> GAMEADLSEPFSLTEVQTAYMLGRNPQFELSGISPQTYFEYETELDIARLSRSFQKVIQRHPMLRAVILPEGKQQILRDVPEYEIEVESLVSMPPEKQAARLREERSRMIDHVFPLGQWPLFELKAFQLQEHTYLLCFRYDALLMDGASMNLVGQDLMHYYHQPDAQLPPLSFTFQDYMHIYDDMKRGTEYETAKAYWTNKLPDFPPAPSLLLAKDPAEIGTPNFQSLTTIITKDKWLKLRRLAQDKQVTPSALLCTVYGEVLAFWSNQRRLAINLTVFNRYPVHDEVEQIVGDFTSLILLDMDMDQKQPFFTKVEQTQSTLLDGLEHRHYDGVEFIRDYTRYHQMRPKAVMPIVFTSMLAGAGAFAWEEIGSLRHIHARTPQVYLDNVVIEKNGELLVSWNYVEELFDAEVMESMFTQFVELLDQLVEQGDINPLRISQKDYALIDQYNATAEPIPAATLHQLFIDQAQRTPDQVAVVFEQEWLTYSELDQRSNQVARFLQSRGIGRGDRVGVLAKRQVETIINLMAVLKAGAAYVPIDPDHPYERQTYILENSSCKILLDSDLYETMEISSYADGDLTPVAEPEDTAYVIYTSGSTGRPKGVIITHQAASNTIQDINRKFEVNEEDRIIGISSMCFDLSVYDIFGTLSAGATLVMIRDPRDMRELVRTVERRGITIWNTVPAIMDLALDHVGSHFENISLRLVLLSGDWIPLPLPAKINRHFPVADVISLGGATEASIWSIYWPIEQVEANWKSIPYGKPLANQTYYVLNYDQKMCPVGVIGDLYIGGAGLAQGYLNDDQKTKDAFIMHPEFGPIYKTGDCGRMRPEGYIEFLGRQDYQVKIQGYRVELEEISHCLLTYPDVDQAVVIDQTDERGMKFLVGYVVAQQEIDEKALRKHLMEHLPEYMIPAHLVHLEQLPLTPNGKLDRKALPVPKKQRNAEKFVAPQAGLEKILASVWQEVLNVEQIGANDHFFALGGDSIKAIQVSARLFVQGYHLDTKSLFEFPVLRDVARTIKKLAAAENLFY;> GAMGEQIFYWSPAKHWRMSDEGVVIGESTYTGMILEWFPEFYFFAQTGVTINRLLERFSSGSEKEANEILELLIQDRVLVEGILPPREVFSPQEGLFVNPYSEQIRYSKEALDYYVSEQLNRTHAACRSTKIQLETSGALPDIIQKRRSCRRFDMKTPVSFATFSNLLSSLKQRKEDKILYNYASAGGLYPIDVFVYVKPRRVEGVKAGFYYFNPADHSLVLVNNIDQVIKDDHELINQDIFAQSAFSVYLVYNARASMPKYGAAGYFYACIEAGIITATLNMVAEDLNVGLCSIGHMNFEEIQTFLKLEDHQVILHAIEGGLKIDGAAAENLFY

The bacillamide biosynthetic pathway is a common, three-protein system, with a decarboxylase that prepares an NRPS substrate, an NRPS, and an oxidase. The oxidase is shown to perform dehydrogenation of the thiazoline in the peptide intermediate while it is covalently attached to the NRPS, as the penultimate step in bacillamide D synthesis. The oxidase forms a stable complex with the NRPS and dimerizes it. We visualized co-complexes of the oxidase bound to the elongation module of the NRPS using X-ray crystallography and cryo-EM.

BmdBM2–BmdC complex is a very elongated dimeric structure in which the two BmdB modules are kept far apart, and in which the active sites accessed by PCP2 form a catalytic arc. The center of the complex is BmdC in the same dimeric configuration described above. The area of the BmdC Ox domain most distal from the dimeric interface (residues 223–231 and 303–306) makes a small interface with one end of the A domain (residues 1321–1323, 1468, 1512–1513), burying 491 Å2 of surface area per protein. This positions the two BmdBM2 modules in a plane perpendicular to the BmdC rotational axis, stretching out at ~45° to the core BmdC dimer interface. The configuration is extremely oblong, with the BmdBM2:BmdC complex having overall dimensions of 65 Å by 65 Å by 280 Å and placing the Cy2 domains on either side of the massive complex. Surprisingly, A2sub is disordered, despite no visible impediment to its binding in its classic thiolation position, suggesting A2sub may not be required to help position PCP2 for aminoacylation. In the catalytic cycle of module 2, PCP2 must visit A2 for thiolation/aminoacylation to ligate the cysteine substrate (forming Cys-S-PCP2), then the Cy2 domain for condensation and heterocyclization (forming AlaCysthiazoline-S-PCP2) and the BmdC Ox domain for oxidation (forming AlaCysthiazole-S-PCP2).> RTPEMPVLENRAAQGDITAPGGARRLTGDQTAALRDSLSDKPAKNIILLIGDGMGDSEITAARNYAEGAGGFFKGIDALPLTGQYTHYALNKKTGKPDYVTDSAASATAWSTGVKTYNGALGVDIHEKDHPTILEMAKAAGLATGNVSTAELQDAVPAALVAHVTSRKCYGPSATSEKCPGNALEKGGKGSITEQLLNARADVTLGGGAKTFAETATAGEWQGKTLREQAQARGYQLVSDAASLNSVTEANQQKPLLGLFADGNMPVRWLGPKATYHGNIDKPAVTCTPNPQRNDSVPTLAQMTDKAIELLSKNEKGFFLQVEGASIDKQDHAANPCGQIGETVDLDEAVQRALEFAKKEGNTLVIVTADHAHASQIVAPDTKAPGLTQALNTKDGAVMVMSYGNSEEDSQEHTGSQLRIAAYGPHAANVVGLTDQTDLFYTMKAALGLKLEHHHHHH;> RTPEMPVLENRAAQGDITAPGGARRLTGDQTAALRDSLSDKPAKNIILLIGDGMGDSEITAARNYAEGAGGFFKGIDALPLTGQYTHY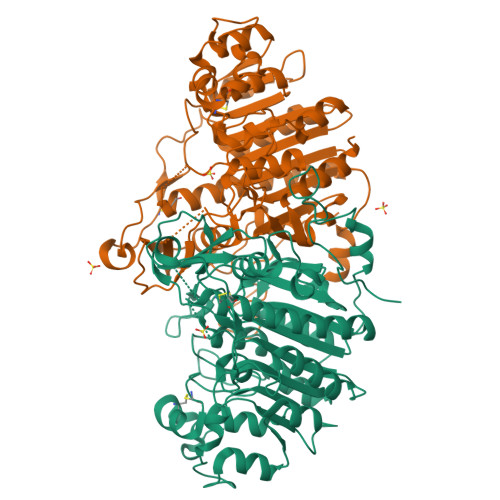ALNKKTGKPDYVTDSAASATAWSTGVKTYNGALGVDIHEKDHPTILEMAKAAGLATGNVSTAELQDATPAALVAHVTSRKCYGPSATSEKCPGNALEKGGKGSITEQLLNARADVTLGGGAKTFAETATAGEWQGKTLREQAQARGYQLVSDAASLNSVTEANQQKPLLGLFADGNMPVRWLGPKATYHGNIDKPAVTCTPNPQRNDSVPTLAQMTDKAIELLSKNEKGFFLQVEGASIDKQDHAANPCGQIGETVDLDEAVQRALEFAKKEGNTLVIVTADHAHASQIVAPDTKAPGLTQALNTKDGAVMVMSYGNSEEDSQEHTGSQLRIAAYGPHAANVVGLTDQTDLFYTMKAALGLKLEEEEEEE>[5x]GSHMKRDSRIYFDITDDVEMNTYNKSKMDKRRDLLKRGFLTLGAQITQFFDTTVTIVITRRSVENIYLLKDTDILSRAKKNYMKVWSYEKAARFLKNLDVDLDHLS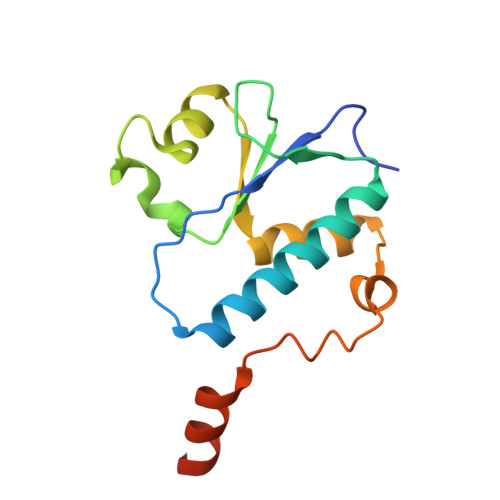KTKSASLAAPTLSNLLHNEKLYGPTDRD> AAP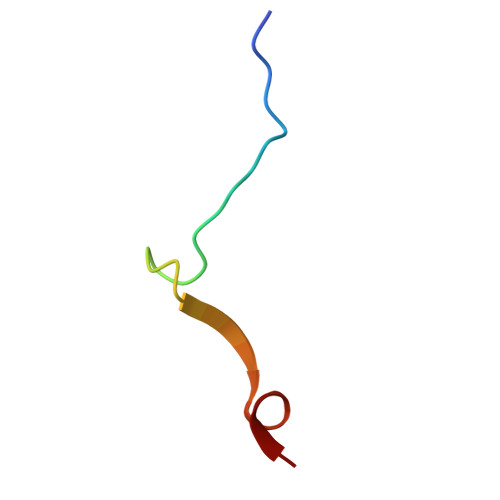VINSHTCFVSGNSNMILNHMNDNFA>AGAGGCCTCT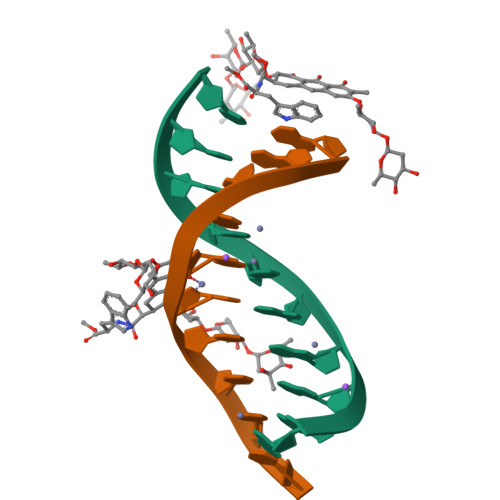[4x]>SQEVMKNLSLNFGKALDECKKEMTLTDAINEDFYNFWKEGYEIKNRETGCAIMCLSTKLNMLDPEGNLHHGNAMEFAKKHGADETMAQQLIDIVHGCEKSTPANDDKCIWTLGVATCFKAEIH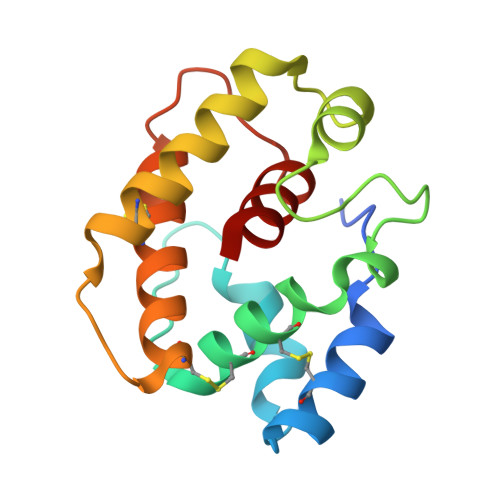KLNWAPSMDVAVGEILAEV[2x]>[6x]MKLEIFSWWAGDEG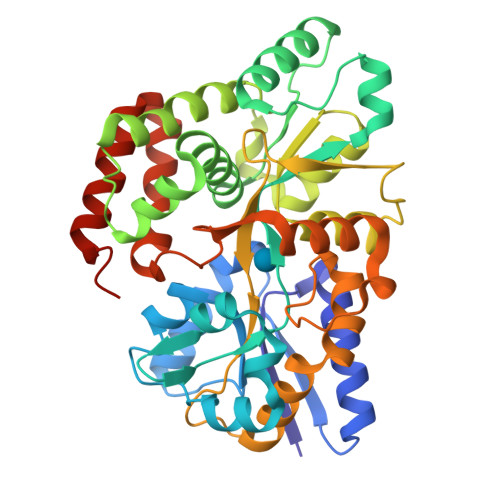PALEALIRLYKQKYPGVEVINATVTGGAGVNARAVLKTRMLGGDPPDTFQVHAGMELIGTWVVANRMEDLSALFRQEGWLQAFPKGLIDLISYKGGIWSVPVNIHRSNVMWYLPAKLKGWGVNPPRTWDKFLATCQTLKQKGLEAPLALGENWTQQHLWESVALAVLGPDDWNNLWNGKLKFTDPKAVRAWEVFGRVLDCANKDAAGLSWQQAVDRVVQGKAAFNIMGDWAAGYMTTTLKLKPGTDFAWAPSPGTQGVFMMLSDSFGLPKGAKNRQNAINWLRLVGSKEGQDTSNPLKGSIAARLDSDPSKYNAYGQSAMRDWRSNRIVGSLVHGAVAPESFMSQFGTVMEIFLQTRNPQAAANAAQAIADQVGLGRLGQHHHHHH>MGEKNGDAKTFWMELEDDGK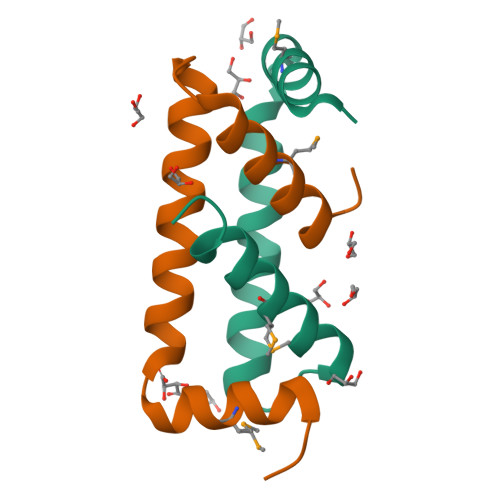VDFIFEQVQNVLQSLKQKIKDGSATNKEYIQAMILVNEATIINS[2x]> AALRERAGPVTWVMMIACVVVFIAMQILGDQEVMLWLAWPFDPTLKFEFWRYFTHALMHFSLMHILFNLLWWWYLGGAVEKRLGSGKLIVITLISALLSGYVQQKFSGPWFGGLSGVVYALMGYVWLRGERDPQSGIYLQRGLIIFALIWIVAGWFDLFGMSMANGAHIAGLAVGLAMAFVDSLNARKRK

Rhomboid intramembrane proteases are evolutionarily conserved proteins with numerous important biological functions, including growth factor secretion, regulation of mitochondrial dynamics, and membrane protein quality control (Fleig et al., 2012). Rhomboids are serine proteases with a Ser-His catalytic dyad (Wang et al., 2006), and they recognize their transmembrane substrates in a two-tier process. It is assumed that first a portion of the transmembrane domain of the substrate docks into an intramembrane interaction site of rhomboid within the plane of the lipid bilayer, upon which a linear segment of the substrate (possibly generated by local unfolding of the top of the substrate's transmembrane helix) interacts with the water-exposed active site (reviewed in Strisovsky, 2016a, Strisovsky, 2013).

To understand why peptidyl ketoamides are such efficient rhomboid inhibitors and to establish the basis for structure-guided design of their improved variants, we determined the co-crystal structures of GlpG with 9 and 10. The complexes were formed by soaking the inhibitors into apoenzyme crystals, and the structures were solved using diffraction data to 2.16 and 1.78 Å resolution, respectively, allowing detailed comparison of their binding modes. In both cases, the pentapeptide RVRHA binds the active site cavity as an extended β strand, virtually identically to the binding mode of Ac-RVRHA-cmk. In both inhibitors, the ketoamide warhead is covalently bonded via its proximal carbon to the side-chain oxygen of the catalytic S201, and it engages in a network of six hydrogen bonds in the active site. The oxyanion formed by the proximal carbonyl oxygen accepts hydrogen bonds from His150 and the main-chain amide nitrogen of the catalytic serine, and the distal ketoamide carbonyl oxygen accepts hydrogen bonds from both H150 and N154, thus amply saturating the hydrogen-bonding groups engaged in the stabilization of the oxyanion (Cho et al., 2016). Furthermore, the ketoamide nitrogen donates a hydrogen bond to H254 and to the S201 side-chain oxygen covalently bound to the warhead. The resulting network of six hydrogen bonds probably helps position the ketoamide warhead in the proximity of the hydroxyl of the catalytic S201 to enhance its chemical reactivity in a conformation-dependent manner. The tail substituents of 9 and 10 (RT9 and RT10) interact with the prime side of GlpG, buried in a cavity delimited by the side chains of amino acids F245, M247, and M249 from the L5 loop, W236 from TMD5, F153 and W157 from TMD2, and residues V204, M208, Y205, H254, H150, and N154.GDP-perosamine 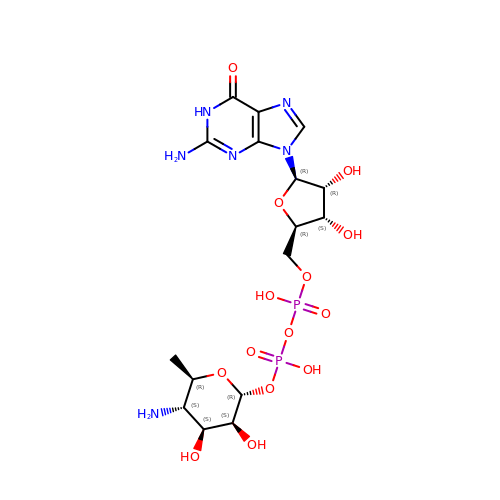| C16 H26 N6 O14 P2 | PMFIPWCEUCAMAY-YVXBHLEUSA-N> MALKMLTRLQVLTLALFSKGFLLSLGDHNFLRREIKIEGDLVLGGLFPINEKGTGTEECGRINEDRGIQRLEAMLFAIDEINKDDYLLPGVKLGVHILDTCSRDTYALEQSLEFVRASLTKVDEAEYMCPDGSYAIQENIPLLIAGVIGGSYSSVSIQVANLLRLFQIPQISYASTSAKLSDKSRYDYFARTVPPDFYQAKAMAEILRFFNWTYVSTVASEGDYGETGIEAFEQEARLRNISIATAEKVGRSNIRKSYDSVIRELLQKPNARVVVLFMRSDDSRELIAAASRANASFTWVASDGWGAQESIIKGSEHVAYGAITLELASQPVRQFDRYFQSLNPYNNHRNPWFRDFWEQKFQCSLQNKRNHRRVCDKHLAIDSSNYEQESKIMFVVNAVYAMAHALHKMQRTLCPNTTKLCDAMKILDGKKLYKDYLLKINFTAPFNPNKDADSIVKFDTFGDGMGRYNVFNFQNVGGKYSYLKVGHWAETLSLD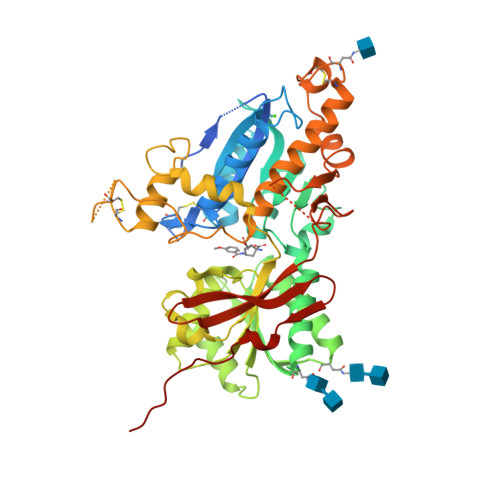VNSIHWSRNSVPTSEGHHHHHH>[2x]MALGSLLALLALLLLWGAVAEGPAKKVLTLEGDLVLGGLFPVHQKGGPAEDCGPVNEHRGIQRLEAMLFALDRINRDPHLLPGVRLGAHILDSCSKDTHALEQALDFVRASLSRGADGSRHICPDGSYATHGDAPTAITGVIGGSYSDVSIQVANLLRL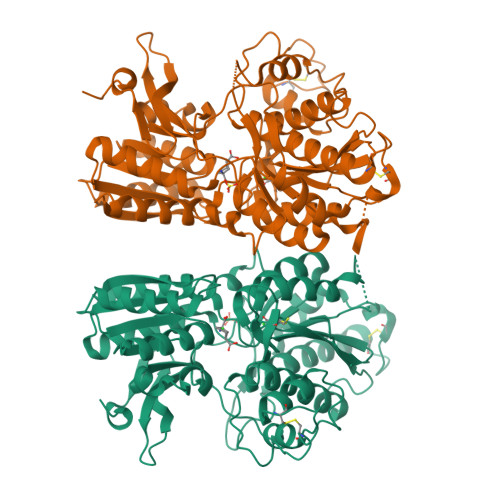FQIPQISYASTSAKLSDKSRYDYFARTVPPDFFQAKAMAEILRFFNWTYVSTVASEGDYGETGIEAFELEARARNISVATSEKVGRAMSRAAFEGVVRALLQKPSARVAVLFTRSEDARELLAASQRLNASFTWVASDGWGALEEVVAGSEGAAEGAITIELASYPISDFASYFQSLDPWNNSRNPWFREFWEQRFRCSFRQRDCAAHSLRAVPFEQESKIMFVVNAVYAMAHALHNMHRALCPNTTRLCDAMRPVNGRRLYKDFVLNVKFDAPFRPADTHNEVRFDRFGDGIGRYNIFTYLRAGSGRYRYQKVGYWAEGLTLDTSLIPWASPSAGEGHHHHHH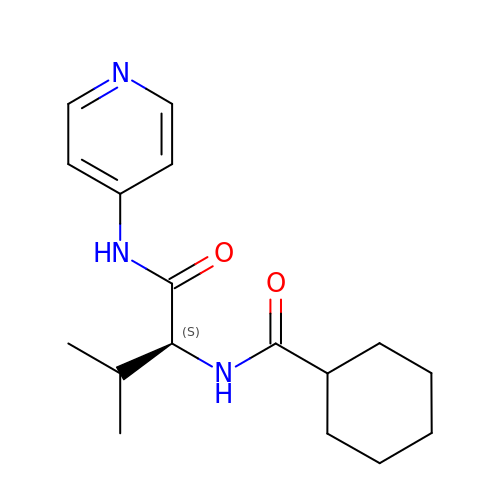N-[(1S)-2-methyl-1-(pyridin-4-ylcarbamoyl)propyl]cyclohexanecarboxamide | C17 H25 N3 O2 | VYLDPSVXLWTIAJ-HNNXBMFYSA-N> NDPITNAVESAVSALADTTISRVTAANTAASTHSLGTGRVPALQAAETGASSNSSDENLIE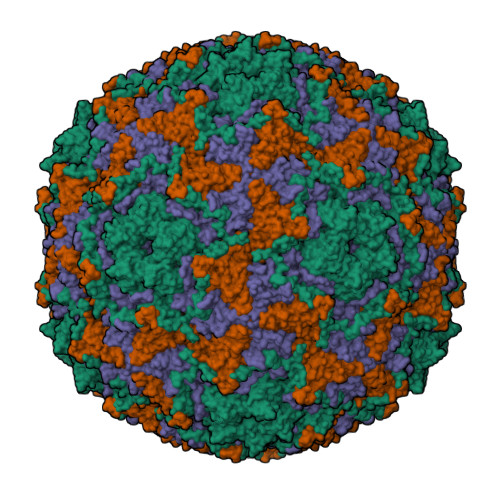TRCVMNRNGVNEASVEHFYSRAGLVGVVEVKDSGTSLDGYTVWPIDVMGFVQQRRKLELSTYMRFDAEFTFVSNLNNSTTPGMLLQYMYVPPGAPKPDSRKSYQWQTATNPSVFAKLSDPPPQVSVPFMSPATAYQWFYDGYPTFGEHKQATNLQYGQCPNNMMGHFAIRTVSESTTGKNIHVRVYMRIKHVRAWVPRPLRSQAYMVKNYPTYSQTITNTATDRASITTTDYEGGVPASPQRTS;> SPSVEACGYSDRVAQLTVGNSTITTQEAANIVLSYGEWPEYCPSTDATAVDKPTRPDVSVNRFYTLSTKSWKTESTGWYWKFPDVLNDTGVFGQNAQFHYLYRSGFCMHVQCNASKFHQGALLVAAIPEFVIAASSPATKPNSQGLYPDFAHTNPGKDGQEFRDPYVLDAGIPLSQALIFPHQWINLRTNNCATIIMPYINALPFDSALNHSNFGLVVIPISPLKYCNGATTEVPITLTIAPLNSEFSGLRQAIKQ;> GFPTELKPGTNQFLTTDDGTSPPILPGFEPTPLIHIPGEFTSLLDLCQVETILEVNNTTGTTGVSRLLIPVRAQNNVDQLCASFQVDPGRNGPWQSTMVGQICRYYTQWSGSLKVTFMFTGSFMATGKMLIAYTPPGSAQPTTREAAMLGTHIVWDFGLQSSVTLVIPWISNTHFRAVKTGGVYDYYATGIVTIWYQTNFVVPPDTPTEANIIALGAAQKNFTLKLCKDTDEIQQTAEYQ;> MGAQVSTQKSGSHETRNVATEGSTINFTNINYYKDSYAASASRQDFAQDPAKFTRPVLDAIREAAAPLQ> HGSVVDPASRSYSCWQRWGGDFQNPAMATQDPMCWQAWQADPNAMWNWNGLFREGVAGNHQGAIPDGQLCSGGRTQSGRYNALDTVGAWKTVPVTNNFRVKFF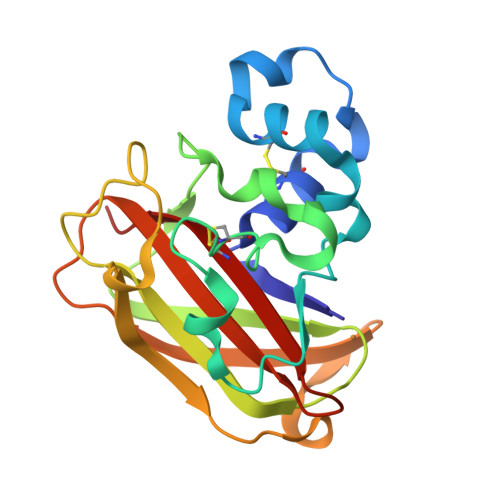DQASHGADYIRVYVTKQGYNALTSPLRWSDLELVGQIGNTPASQWTREVDGVSIQIPANAPGRTGRHVVYTIWQASHLDQSYYLCSDVDFG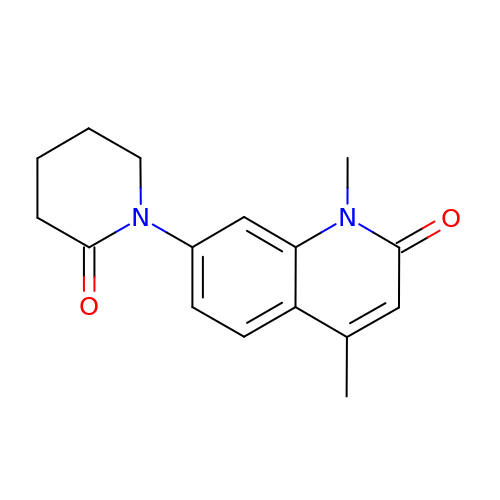1,4-dimethyl-7-(2-oxopiperidin-1-yl)quinolin-2(1H)-one | C16 H18 N2 O2 | TVJZEYRKRPKMHK-UHFFFAOYSA-N The hLL-3717–29 fragment was suggested to serve as the active core of the AMP, showing a different spectrum of antibacterial activity as compared to the full-length protein and other fragments, including being the shortest LL-37 fragment retaining anti-viral activity. Here we demonstrate that the active core peptide of hLL-37, containing residues 17–19 (hLL-3717–29), formed supra-helical highly stable fibrils that interact with bacterial cells. Rather, the fibrillar assembly of LL-3717–29 was comprised of associating four-helix bundles, each stabilized by a closely packed hydrophobic core. To conclude, the atomic structures of human and primate antibacterial LL-3717-29 showed a functional supramolecular nanostructure of densely packed amphipathic helices.

The gorilla LL-37 (gLL-37) sequence contains two amino acid substitutions when compared to hLL-37, with one at position 17, the first residue of LL-3717-29, substituting phenylalanine with serine (corresponding to a F17S mutation). gLL-3717-29 exhibited slightly weaker antibacterial activity against M. luteus compared to hLL-3717-29, with a MIC of 53 µM, similar to the effect of the F17A mutant. The 1.1 Å resolution crystal structure of gLL-3717-29 displayed a similar assembly compared to hLL-3717-29, with almost identical backbone positions and root-mean-square deviation (RMSD) of 0.15 Å, differing only in the two N-terminal positions that lined the central pore. The overall structure of the two is highly similar (RMSD of 0.15 Å for the asymmetric unit, comprising two helices and a similar space group and unit cell dimensions). The N-termini of the helices, with Phe17 in hLL-3717-29 or Ser17 in gLL-3717-29, and Lys18, line the central pore. The pore of gLL-3717-29 is more occluded, due to the orientation of the lysine residues extending into the pore. Similarly, the mean MIC value gLL-3717-29 (equivalent to an F17S mutation) is 53 µM.

>[2x]SKRIVQRIKDFLR6-(dimethylamino)-8-fluoro-2-[2-(hydroxymethyl)-3-(1-methyl-5-{[5-(morpholin-4-ylcarbonyl)pyridin-2-yl]amino}-6-oxo-1,6-dihydropyridin-3-yl)phenyl]isoquinolin-1(2H)-one 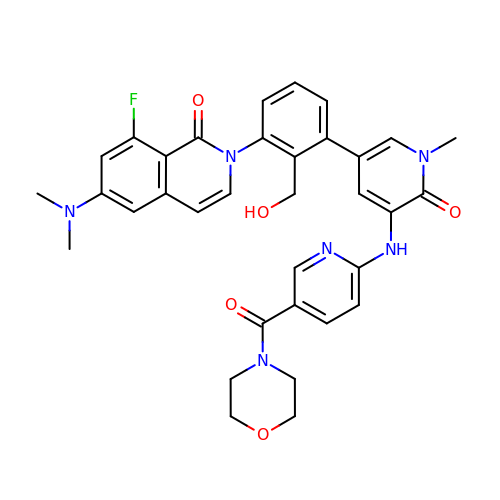| C34 H33 F N6 O5 | PCVMXQPADBQRFE-UHFFFAOYSA-N>MIVRNLGDIRKTDRNVRSDGWASARMLLKDDGMGFSFHVTTLFAGSELRMHYQNHLEAVLVLKGTGTIEDLATGEVHALRPGVMYALDDHDRHIVRPETDILTACVFNPPVTGREVHDESGAYPADPELAREPVAADNWSHPQFEK[4x]

Each of these enzymes catalyzes as their main activity the cyclization of N-γ-acetyl-L-2,4-diaminobutyric acid (N-γ-ADABA), the reaction product of the 2,4-diaminobutyrate acetyltransferase (EctA), to ectoine with the concomitant release of a water molecule. We demonstrate here for the first time that the ectoine synthase is a metal-dependent enzyme, with iron as the most likely physiologically relevant co-factor. The EctC protein forms a dimer in solution and our structural analysis identifies it as a member of the cupin superfamily. The two crystal structures that we report here for the (Sa)EctC protein (with resolutions of 1.2 Å and 2.0 Å, respectively), and data derived from extensive site-directed mutagenesis experiments targeting evolutionarily highly conserved residues within the extended EctC protein family, provide a first view into the architecture of the catalytic core of the ectoine synthase.

The second crystal structure of the (Sa)EctC protein was solved at a resolution of 2.0 Å and contained four molecules of the protein in the asymmetric unit of which protomer A comprised amino acid Met-1 to Gly-121 and adopts a closed conformation. We therefore cannot exclude that this crystal structure does not represent the fully closed state of the ectoine synthase; consequently, we tentatively termed it the “semi-closed” (Sa)EctC structure. In the “semi-closed” structure, a longer carboxy-terminal tail is visible in the electron density, folding into a small helix (α-II) that closes the active site of the (Sa)EctC protein. The formation of this α-II helix induces a reorientation and shift of a long unstructured loop (as observed in the “open” structure) connecting β4 and β6, resulting in the formation of the stable β-strand β5 as observed in the “semi-closed”state of the (Sa)EctC protein. In the “semi-closed” crystal structure, (Sa)EctC has crystallized as a dimer of dimers within the asymmetric unit. This dimer is composed of two monomers arranged in a head-to-tail orientation and is stabilized via strong interactions mediated by two antiparallel β-strands, β-strand β1 (sequence 1MIVRN5) from monomer A and β-strand β8 from monomer B (sequence 82GVMYAL87). In the “semi-closed” structure of (Sa)EctC, each of the four monomers in the asymmetric unit contains a relative strong electron density positioned within the cupin barrel. Only the refinement of Fe2+ resulted in a visibly improved electron density, however with a low degree of occupancy. This possible iron molecule is bound via interactions with Glu-57, Tyr-85 and His-93. Since both the refinement and the distance did not clearly identify an iron molecule, we decided to conservatively place a water molecule at this position. However, in the “semi-closed” (Sa)EctC structure where the carboxy-terminal loop is largely resolved, a long stretched electron density feature was detected in the predicted active site of the enzyme; it remained visible after crystallographic refinement.> MQRSPLEKANIFSKLFFRWTKPILKKGYRQRLELSDIYQIPSADSADNLSEKLEREWDRELATSKKKPKLINALRRCFFWKFMFYGILLYLGEVTKSVQPLLLGRIIASYDPDNSSERSIAYYLGIGLCLLFLVRTLLIHPSIFGLHHIGMQIRI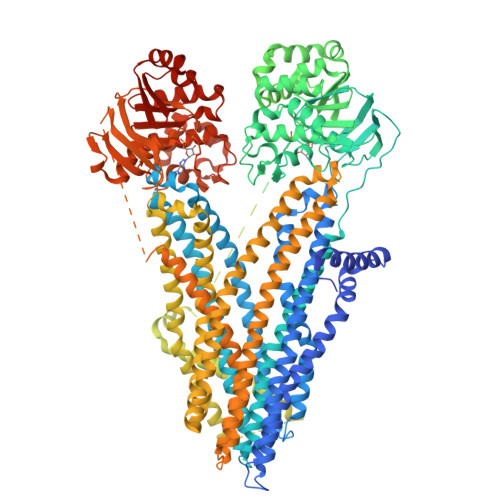ALFSLIYKKTLKLSSKVLDKISTGQLVSLLSNNLNKFDEGLALAHFVWIAPLQVALLMGLLWDMLQASAFAGLAFLIVMAFFQAWLGQMMMKYRDKRAGKINERLVITSEIIENIQSVKAYCWEDAMEKMIESLRETELKLTRKAAYVRYFNSSAFFFSGFFVVFLAVVPYAVTKGIILRKIFTTISFCIVLRMTVTRQFPGSVQTWYDSIGAINKIQDFLLKEEYKALEYNLTTTGVEVDKVTAFWDEHASPVLQDINFKIEKGELLAVSGSTGSGKTSLLMLIMGELEPSEGKIKHSGRISFSPQVSWIMPGTIKENIIFGVSYDEYRYKSVIQACQLEEDILKFPDKDYTVLGEGGIILSGGQRARISLARAVYKDADLYLMDSPFGYLDIFTEKEIFESCVCKLMANKTRILVTSKLEHLKIADKILILHEGSCYFYGTFSELQGQRPDFSSELMGFDSFDQFSAERRNSIITETLRRFSFEGESMGSRNEMKKQSFKQTSDFNDKRKNSIIINPLNAGRKLSIMQKNGTQVNGLEDGHIDSPERRISLVPDLEQGDVGLPRSNMLNSDHMLQSRRRQSVLSLMTGTSVNQGPHVSKKGSTSFRKMSVVPQTNLSSEIDIYTRRLSRDSILDITDEINEEDLKECFTDDAESMGTVTTWNTYFRYITIHKSLIFVLILCVTIFLLEVAASLVLLLFLQKAAQINATQPENATSDNPPVIITDTSSYYMIYIYVGIADTLLAMGIFRGLPLVHTLITVSKTLHQKMVHAVLYAPMSTFNSLKAGGILNRFSKDTAILDDLLPLTVFDLIQLILIVIGAITVVSILQPYIFLASVPVIAAFIVLRAYFLHTSQQLKQLESEARSPIFTHLVTSLKGLWTLRAFGRQPYFETLFHKALNLHTANWFLYLSTLRWFQMRIEMIFVVFFSAVAFISIITTGDGPGRVGIILTLAMNIMGTLQWAVNSSIDVDSLMRSVSRIFKFIDMPTEEMKTIKPQKNNQFSDALIIENRHVKDEKNWPSGGQMTVTDLTARYTEGGTAVLENISFSISSGQTVGLLGRTGSGKSTLLFAFLRLLNTEGDIQIDGVSWNTVSLQQWRKAFGVIPQKVFIFSGTFRKNLDPYGQWNDEEIWKVAEEVGLKSVIEQFPGQLDFVLVDGGCVLSHGHKQLMCLARSVLSKAKILLLDEPSAHLDPITSQVIRKTLKHAFADCTVVLSESRLEAILECQRFLVIEDNKMRQYESIQKLLSEKSSLRQSGSGGGGGGSLEVLFQGDHHHHHHHHHH[[[2-AMINO-5,6,7,8-TETRAHYDRO-4-HYDROXY-PYRIDO[2,3-D]PYRIMIDIN-6-YL]-ETHYL]-PHENYL]-CARBONYL-GLUTAMIC 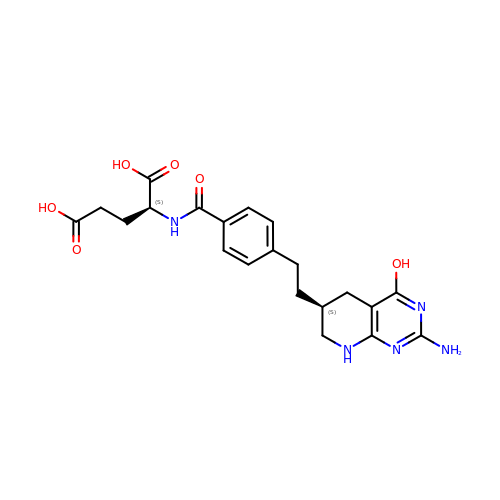ACID | C21 H25 N5 O6 | ZUQBAQVRAURMCL-WFASDCNBSA-N> QDADKLPHTKVTLVAPPQVHPHEQATKSGPKVVEFTMTIEEKKMVIDDKGTTLQAMTFNGSMPGPTLVVHEGDYVQLTLVNPATNAMPHNVDFHGATGALGGAKLTNVNPGEQATLRFKADRSGTFVYHCAPEGMVPWHVVSGLSGTLMVLPRDGLKDPEGKPLHYDRAYTIGEFDLYIPKGPDGKYKDYATLAESYGDTVQVMRTLTPSHIVFNGKVGALTGANALTAKVGETVLLIHSQANRDTR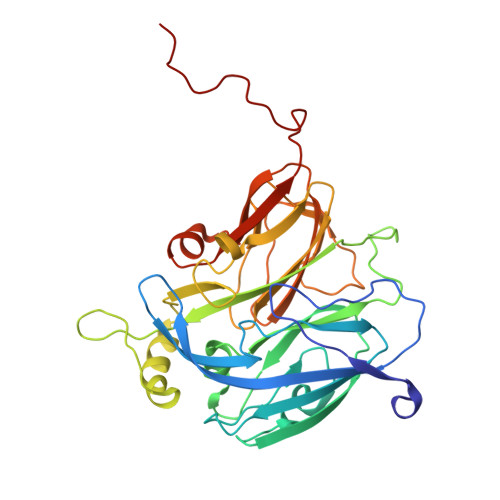PHLIGGHGDWVWETGKFANPPQRDLETWFIRGGSAGAALYTFKQPGVYAYLNHNLIEAFELGAAGHIKVEGKWNDDLMKQIKAPAPIPR> GSTGSDNQYKFKLKNITDSVEQALKIAKQIKDDLDIIEFHRIKLSNHYGIRAEEHEKQTAREELSKFSKDKLEADLKKLLSEIEKSLNAATILITYNDYGGNLQ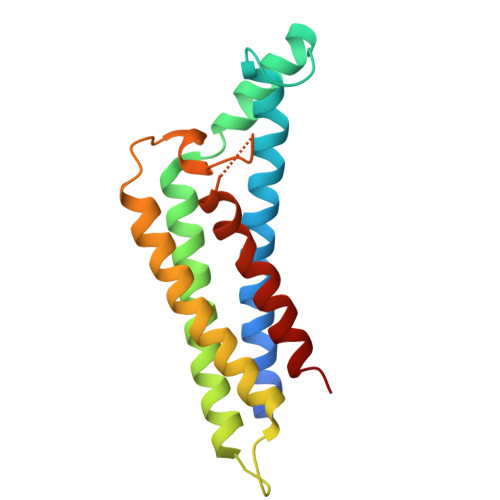SDLSAKTTLEALKTEVSSLITKIQDFNNKDHQAYPTSYYNDYQTYQALRNPYSKLTLVKDLLTRT> MTVKAPSVTSLRISKLSANQVQVRWDDVGANFYYFVEIAETKTNSGENLPSNQYRWINLGYTANNSFFFDDADPLT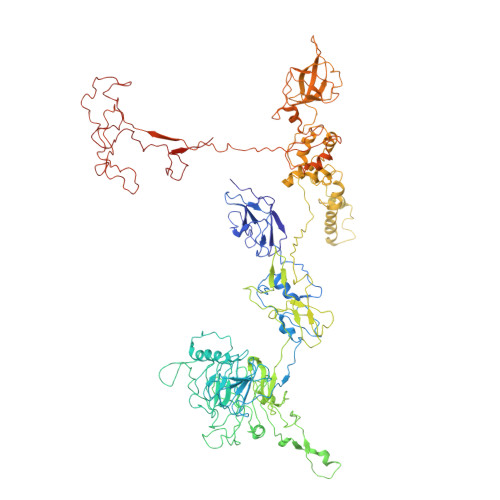TYIIRVATAAQDFEQSDWIYTEEFETFATNAYTFQNMIEMQLANKFIQEKFTLNNSDYVNFNNDTIMAALMNESFQFSPSYVDVSSISNFIIGENEYHEIQGSIQQVCKDINRVYLMESEGILYLFERYQPVVKVSNDKGQTWKAVKLFNDRVGYPLSKTVYYQSANTTYVLGYDKIFYGRKSTDVRWSADDVRFSSQDITFAKLGDQLHLGFDVEIFATYATLPANVYRIAEAITCTDDYIYVVARDKVRYIKTSNALIDFDPLSPTYSERLFEPDTMTITGNPKAVCYKMDSICDKVFALIIGEVETLNANPRTSKIIDSADKGIYVLNHDEKTWKRVFGNTEEERRRIQPGYANMSTDGKLVSLSSSNFKFLSDNVVNDPETAAKYQLIGAVKYEFPREWLADKHYHMMAFIADETSDWETFTPQPMKYYAEPFFNWSKKSNTRCWINNSDRAVVVYADLKYTKVIENIPETSPDRLVHEYWDDGDCTIVMPNVKFTGFKKYASGMLFYKASGEIISYYDFNYRVRDTVEIIWKPTEVFLKAFLQNQEHETPWSPEEERGLADPDLRPLIGTMMPDSYLLQDSNFEAFCEAYIQYLSDGYGTQYNNLRNLIRNQYPREEHAWEYLWSEIYKRNIYLNADKRDAVARFFESRSYDFYSTKGIEASYKFLFKVLYNEEVEIEIESGAGTEYDIIVQSDSLTEDLVGQTIYTATGRCNVTYIERSYSNGKLQWTVTIHNLLGRLIAGQEVKAERLPSFEGEIIRGVKGKDLLQNNIDYINRSRSYYVMKIKSNLPSSRWKSDVIRFVHPVGFGFIAITLLTMFINVGLTLKHTETIINKYKNYKWDSGLPTEYADRIAKLTPTGEIEHDSVTGEAIYEPGPMAGVKYPLPDDYNAENNNSIFQGQLPSERRKLMSPLFDASGTTFAQFRDLVNKRLKDNIGNPRDPENPTQVKIDE OphP is an essential enzyme for the biosynthesis of the macrocyclic peptide natural product omphalotin A. The enzyme has been proposed to proteolytically release a peptide intermediate from the precursor protein OphMA and to macrocyclize the multiply α-N-methylated core of this intermediate to produce omphalotin A. Our *in vitro* experiments demonstrate that OphP does not process OphMA but shows robust macrocyclase activity on pre-processed α-N-methylated peptides. OphP tolerates sequence promiscuity in the substrate but has a preference for highly α-N-methylated substrates and for N-methylated glycine residue at the catalytic site. The promiscuity of OphP is explained by structural analysis of co-complexes which reveals a predominantly hydrophobic substrate binding cleft with few interactions between substrate side chains and OphP. Similar to other POPs, the monomer has two domains, an α/β hydrolase domain (residues 1–82, 453–738) and the seven-bladed β-propeller domain (residues 83–452) ([Fig fig4]).

We first determined the structure of the putatively catalytically inactive OphP variant S580A. The eight monomers differ only in flexible loops some of which are involved in crystal contacts. All the monomers in the asymmetric unit adopt a “closed” conformation with the two domains packed against each other. Structure alignment between OphP and GmPOPB confirmed the putative catalytic triad with some deviations regarding the position of its histidine residue ([Fig fig4]). His701 of OphP sits in a flexible loop region (Leu697–Thr707) which is only resolved in two chains (chain A and chain H) where it adopts different conformations (**Figure S11**). Although chain A and H have different arrangements of this loop, in both His701 is around 15 Å away from Ser580 and a structural re-arrangement is required to form the canonical catalytic triad. Apo S580A crystallized in a closed conformation in the absence of ligand ([Fig fig4]).

>[8x]MSFPGWGPYPPVERDETSAITYSSKLHGSVTVRDPYSQLEVPFEDSEETKAFVHSQRKFARTYLDENPDREAWLETLKKSWNYRRFSALKPESDGHYYFEYNDGLQSQLSLYRVRMGEEDTVLTESGPGGELFFNPNLLSLDGNAALTGFVMSPCGNYWAYGVSEHGSDWMSIYVRKTSSPHLPSQERGKDPGRMNDKIRHVRFFIVSWTSDSKGFFYSRYPPEDDEGKGNAPAMNCMVYYHRIGEDQESDVLVHEDPEHPFWISSVQLTPSGRYILFAASRDASHTQLVKIADLHENDIGTNMKWKNLHDPWEARFTIVGDEGSKIYFMTNLKAKNYKVATFDANHPDEGLTTLIAEDPNAFLVSASIHAQDKLLLVYLRNASHEIHIRDLTTGKPLGRIFEDLLGQFMVSGRRQDNDIFVLFSSFLSPGTVYRYTFGEEKGYRSLFRAISIPGLNLDDFMTESVFYPSKDGTSVHMFITRPKDVLLDGTSPVLQYGYGGFSLAMLPTFSLSTLLFCKIYRAIYAIPNIRGGSEYGESWHREGMLDKKQNVFDDFNAATEWLIANKYASKDRIAIRGGANGGVLTTACANQAPGLYRCVITIEGIIDMLRFPKFTFGASWRSEYGDPEDPEDFDFIFKYSPYHNIPPPGDTVMPAMLFFTAAYDDRVSPLHTFKHVAALQHNFPKGPNPCLMRIDLNSGHFAGKSTQEMLEETADEYSFIGKSMGLTMQTQGSVDSSRWSCVTV>[2x]NLEMEIILTLSQGLKKYYGKILKLLHLTLEEDTEGLLEWCKRNLGSNCDDDFFQKRIEEFFITGEGYFNEVLQFKTLSTPSSTEPSHARLPTAEPFKSYFAKGFLSIDSGYFSAKCYPRSSTSGLQLINVTQHPARIAETPGPKTTSLKTINCINLRASVFKEHREVEINVLLPQIAVNLSNCHVVINSHVCDYSLDTDGPVRLPRIYHEGTFMPGTYKIVIDRKNKLNDRCTLVTNCV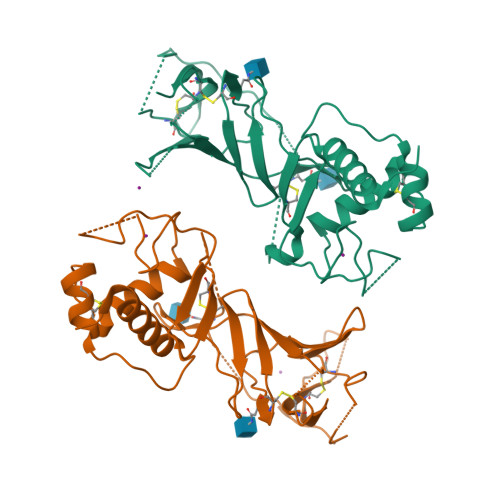IKGREVRKGQSVLRQYKTEIKIGKAPTGSLEVLFQ> GSTREPEIASSLIKQIFSHYVKTPVTRDAYKIVEKCSERYFKQISSDLEAYSQHAGRK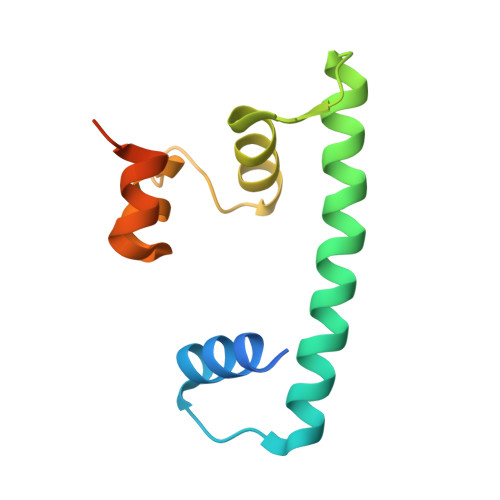TVEMADVELLMRRQGLVTDKMPLHVLVERHLPLEYRKLLIPIAVSGNKVIPCK>GKEQPQVRGELEETQETQEDGNSTQRTTPVSVNYHFTRQCNYKCGFCFHTAKTSFVLPLEEAKRGLLLLKQAGLEKINFSGGEPFLQDRGEYLGKLVRFCKEELALPSVSIVSNGSLIRERWFKDYGEYLDILAISCDSFDEQVNALIGRGQGKKNHVENLQKLRRWCRDYKVAFKIN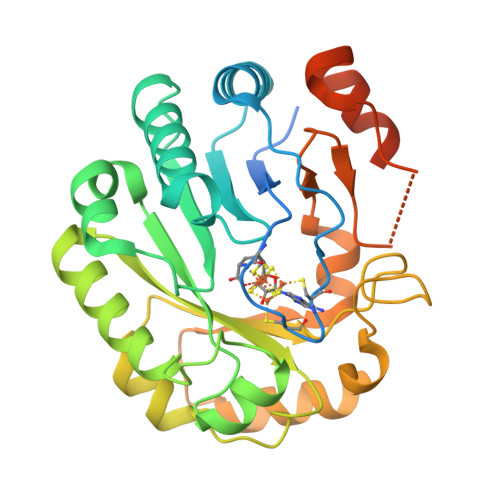SVINRFNVDEDMNEHIKALSPVRWKVFQCLLIEGENSGEDALREAERFLISNEEFETFLERHKEVSCLVPESNQKMKDSYLILDEYMRFLNCTGGRKDPSKSILDVGVEEAIKFSGFDEKMFLKRGGKYVWSKADLKLDW[2x]> VKNPSLICAPVMADSIDKMVIETSKAHELGADLVEIRLDWLKDFNPLEDLKTIIKKSPLPTLFTYRPKWEGGQYEGDENERRDVLRLAMELGADYIDVELQVASEFIKSIDGKKPGKFKVIVSSHNYQNTPSVEDLDGLVARIQQTGADIVKIATTAVDIADVARMFHITSKAQVPTIGLVMGERGLMSRILCSKFGGYLTFGTLDSSKVSAPGQPTIKDLLDLYNFRRIGPDTKVYGIIGKPVSHSKSPIVHNQAFKSVDFNGVYVHLLVDNLVSFLQAYSSSDFAGFSCGIPHKEAALQCCDEVDPLAKSIGAVNTILRRKSDGKLLGYNTDCIGSISAIEDGLRSSGDPSSVPSSSSPLASKTVVVIGAGGAGKALAYGAKEKGAKVVIANRTYERALELAEAIGGKALSLTDLDNYHPEDGMVLANTTSMGMQPNVEETPISKDALKHYALVFDAVYTPRITRLLREAEESGAITVSGSEMFVRQAYEQFEIFTGLPA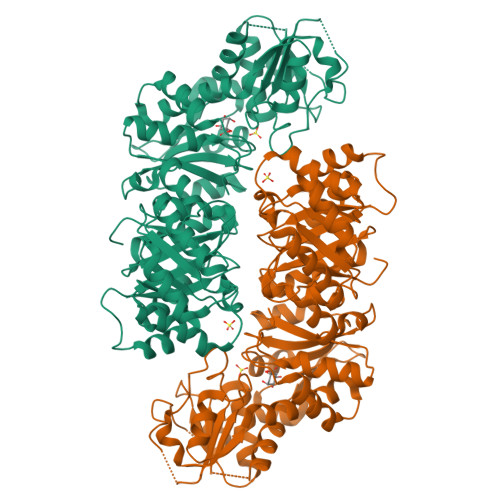PKELYWQIMSKYGSRENLYFQ>[3x]SLNTFYDVQQLLKTFGHIVYFGDRELEIEFMLDELKELY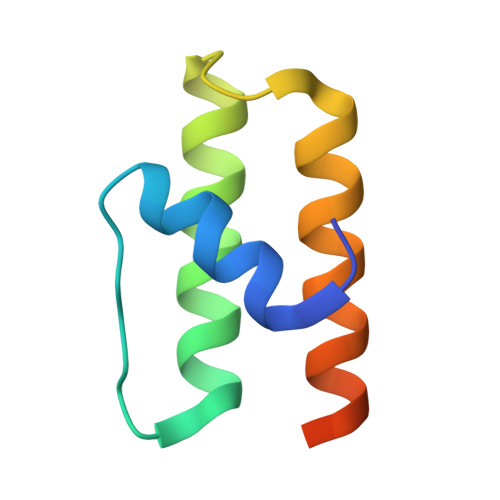MNHMIEKEQWARAAAVLRKELEQTKNGRDFYKG> GPHMGLQESFGVAAEDKIFGGSGSFIPRCMEAMKGVRSMLQCMADKANARNMLQQASLVRPLDNQETLDFSRLSLVEQHECLASILHAAVQRHHATIADFQDFIKILRKWDKYDHFLIHLIPVLAAYITEFGSPEGMGDLQQARRLNDFICKGGDEDSWALPVLGAAVRAWWIAEHNGFYLDDTVQDLRGINLDEEDEQRTKQFLDALKEGAFDFILSVAADCKAQEWQDPSQLGARQWLQRKIPSLPSEPFPFSHFLQHSLMVHLEGFVDATISNLPDVLRKLRTEEDEQRQLRPNHEQDMDLERFLIIISYAYEGRPDAAMSFWEDPDSNLAGFLQWASRRASTPLVSAFCEMLRCLADNEECATAAHNFLLDEGHQASGKMKRSQSLTWSQIFKELEYFTTKVCSERPNPPQASMHRPGRPGADPAEIEPESALMLECYLRLIAKLATESEIARKRLIMDEDFNLVDTILKLSVGVIPHRLRACIFYVLKALMIRKTHEELDAMWRWVEAWMTNPFSSLPGSQGAPQRISFLGQTPGPQECMEMMFREFGTGFEQSNAFIQLLTTLLVPPEGLNSLNDSVPFPEWLGSSIRTLGIEPYVDFVFDVFANRTKDISDPSQLRILRLSCLDFVMVCLVTFNEDLIVLGHESNISIDDAMAATNLATYVRLHPFSRVMEWLFNEKVITSLINTIHQDPISLGSASPDSPLVVSILRAIQVMIKALELQETYLHLVRPEVLRYQGEAGVRRKPVANA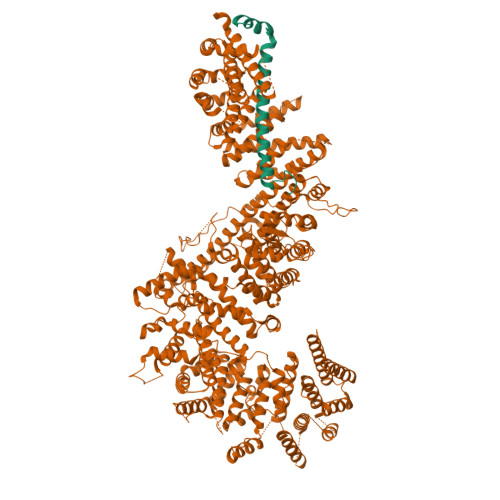AYSAFEDGILSHLSLVVDLGKYCNLGHAELTLACLKLLEKISTSSRILSAWSPDSGRLGHRNKAIVQLERNGEGETISASLSASIMATLDPALAASGENYRVKLAILDFLYACLRATPDQPTIAHQLLGFHCELSKLGIEPKGPFDMQKSLFHSLLNVLITLTVSEEEQGMRGYLVTLKYRVLRILQLLWKSPLSASLVMDELRATNFLFHMLLREVQIQPQLPWDGQLVTGCEFLLSDASLAYIDYLASRAAIFEYIGKELCSVSQNRIPSIKRQIFDALNGQIFVDEEAPLTIPSIFDFFDFINTDYKWEEIPSPHFTYLKDLDLGPCILEHKYAGVHYDIRKAQEILALKRKEYEHSQLATPEFLETVELEEKVLIEWLTVRNRANLLLTARLNLLQAWANLLLVMIESNDFKSTPKMAFLLQALQAILPTLEAFSSLKSDEAFELARVAKVLLWKLDFSQDSDAGLDREQFTVGNLIGDKLFQLFQLCLSAISQCSGTPELRSLYYSICYRYLTAVVDNDATVAATPASSTIGPTRSVTNARARTLKAITLYGDRLLNVICDDAYGSDTTCQTAAMILLNALVHTSRASSAAGVSPADVDCPIIDALNRLNFIGVLVDSLKEILNEWLAPSSTFDPSLSTNASPSLPIPASPSQQYTSAKLALLLQLCQTRQGAKYVLQANLFRALEQSGVFAADPELVEVDSESGVPRVVALERHYALLVALARVVGAAVTARGAHNIVQGRKFLTQHRGLVVHVLKKNAGIGGGVVGNSLASSINGGSTATMTRRDEILAQQALEERIEELAEAFMLLITATGFLEYESEQVPSEQPRAHTTFFH;> SEPGKAHYFLAASGVDPGAAVRDLGALGLQAKTERTAASVGPAAGPSGVSTTGFGTGLGEVDVDTYLSNLQTKTTLSMIADGLERSARDFDAFLEENVTLEWEAQRKRIYQHFGIK(2R,4R)-4-[[(2S,4S)-4-fluoranylpyrrolidin-2-yl]carbonylamino]-1-(2-methylpropanoyl)-N-[[4-[2-[4-(morpholin-4-ylmethyl)phenyl]ethynyl]phenyl]methyl]pyrrolidine-2-carboxamide | C34 H42 F N5 O4 | 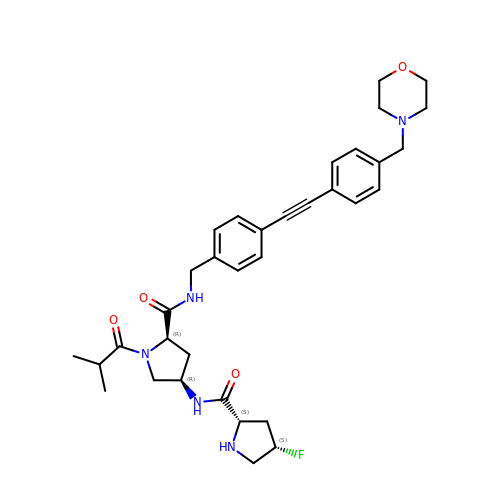HYTBTNOBIMGVDD-XFBWMNOSSA-N>MKALTARQQEVFDLIRDHISQTGMPPTRAEIAQRLGFRSPNAAEEHLKALARKGVIEIVSGASRGIRLLQEEEEGLPLVGRVAADEPLLAQQHIEGHYQVDPSLFKPN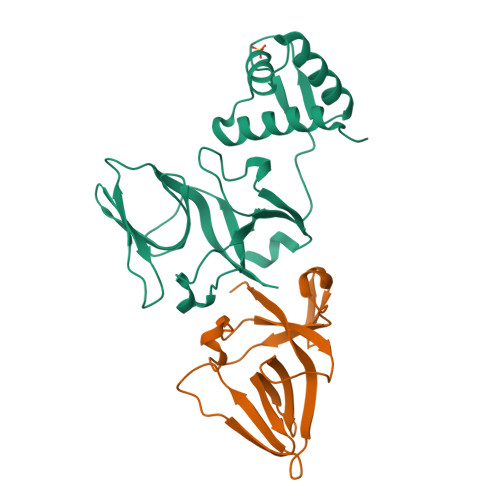ADFLLRVSGMSMKDIGIMDGDLLAVHKTQDVRNGQVVVARIDDEVTVKRLKKQGNKVELLPENSEFKPIVVDLRQQSFTIEGLAVGVIRNGDWL[2x]> MAEKKLEENPYDLDAWSILIREAQNQPIDKARKTYERLVAQFPSSGRFWKLYIEAEIKAKNYDKVEKLFQRCLMKVLHIDLWKCYLSYVRETKGKLPSYKEKMAQAYDFALDKIGMEIMSYQIWVDYINFLKGVEAVGSYAENQRITAVRRVYQRGCVNPMINIEQLWRDYNKYEEGINIHLAKKMIEDRSRDYMNARRVAKEYETVMKGLDRNAPSVPPQNTPQEAQQVDMWKKYIQWEKSNPLRTEDQTLITKRVMFAYEQCLLVLGHHPDIWYEAAQYLEQSSKLLAEKGDMNNAKLFSDEAANIYERAISTLLKKNMLLYFAYADYEESRMKYEKVHSIYNRLLAIEDIDPTLVYIQYMKFARRAEGIKSGRMIFKKAREDARTRHHVYVTAALMEYYCSKDKSVAFKIFELGLKKYGDI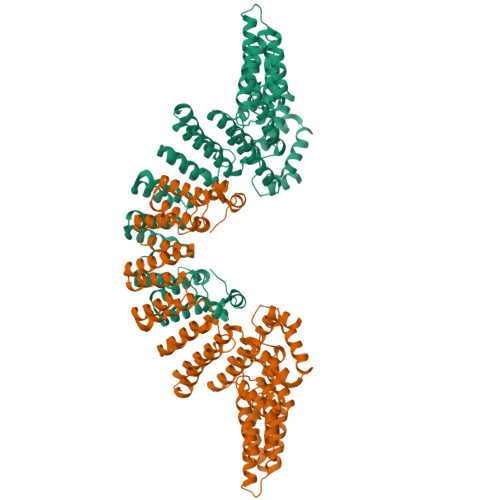PEYVLAYIDYLSHLNEDNNTRVLFERVLTSGSLPPEKSGEIWARFLAFESNIGDLASILKVEKRRFTAFREEYEGKETALLVDRYKFMDLYPCSASELKALGYKDV> GAMGSEKSPSAQELKEQGNRLFVGRKYPEAAACYGRAITRNPLVAVYYTNRALCYLKMQQHEQALADCRRALELDGQSVKAHFFLGQCQLEMESYDEAIANLQRAYSLAKEQRLNFGDDIPSALRIAKKKRWNS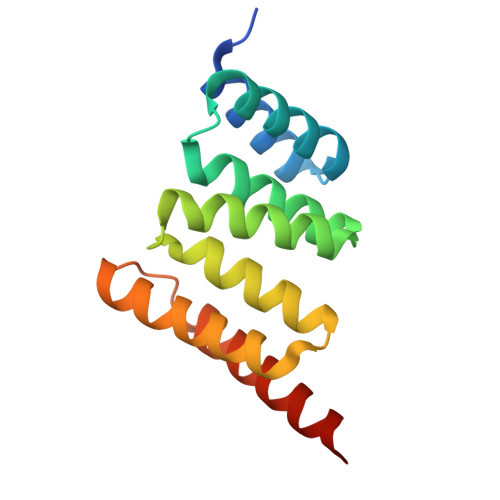IEERR2-[2-[carboxymethyl-[(2-hydroxyphenyl)methyl]amino]ethyl-[(2-hydroxyphenyl)methyl]amino]ethanoic acid | C20 H24 N2 O6 | 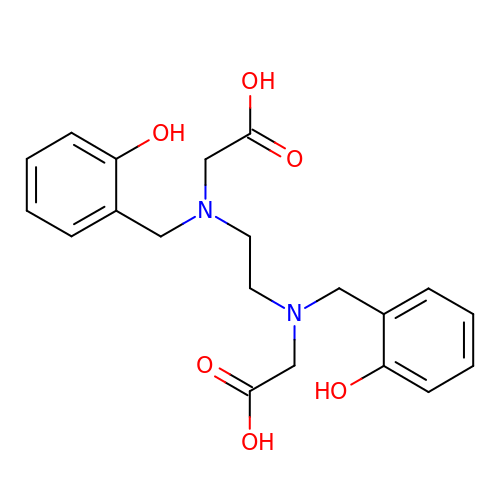GRUVVLWKPGIYEG-UHFFFAOYSA-N6-fluoro-2-[2-methyl-4-phenoxy-5-(propan-2-yl)phenyl]quinoline-4-carboxylic acid | C26 H22 F N O3 | 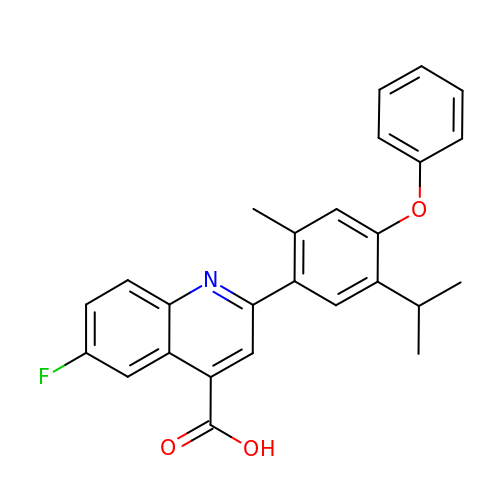KOLKCHJGWGJCTG-UHFFFAOYSA-N> MPCSCASGCQKSKNGGSTPSIRDHVADYYGKTLQSSADLKTSACKLAAAVPESHRKILADIADEVLEKFYGCGSTLPADGSLEGATVLDLGCGTGRDVYLASKLVGEHGKVIGVDMLDNQLEVARKYVEYHAEKFFGSPSRSNVRFLKGFIENLATAEPEGVPDSSVDIVISNCVCNLSTNKLALFKEIHRVLRDGGELYFSDVYADRRLSEAAQQDPILYGECLGGALYLEDFRRLVAEAGFRDVRLVSVGPVDVSDPQLRKLVPDVQFYSCTFRCFKVATLEATREDYGQSATYLGGIGEEFKLDRFFTFPREKPVRVDRNTAEIIRHSRLHQWFSVSAEQQHMGLFKANDS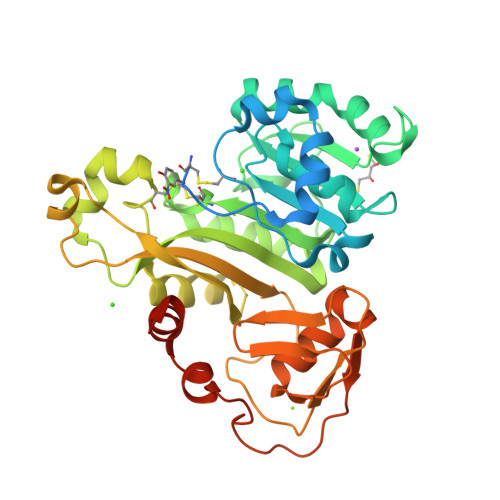YALLHAPLSMQVEQLVSGAAALEHHHHHH> MNNTEENIDRIQEPTREDIDRKEAERLLDEAFNPRTKPVDRKKIINSALKILIGLYKEKKDDLTSASFISIARAYYLVSITILPKGTTIPEKKKEALRKGIEFIDRAINKFNGSILDSQRAFRIKSVLSIEFNRIDREKCDNIKLKNLLNEAVDKGCTDFDTYEWDIQIAIRLCELGVDMEGHFDNLIKSNKANDLQKAKAYYFIKKDDHKAKEHMDKCTASLKYTPCSHRLWDETVGFIERLKGDSSTLWRDFAIKTYRSCRVQEKETGTLRLRWYWSRHRVLYDMAFLAV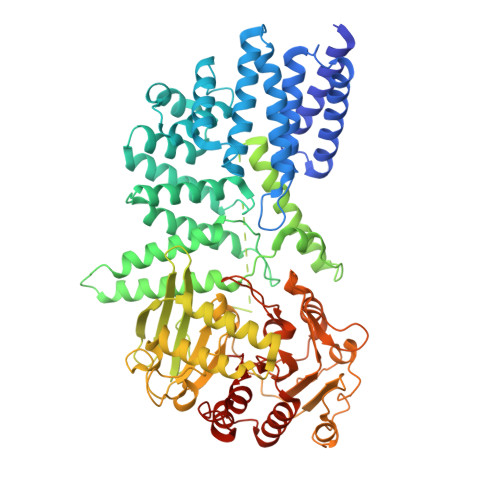KEQADDEEPDVNVKQAKIKKLAEISDSLKSRFSLRLSDMEKMPKSDDESNHEFKKFLDKCVTAYQDGYVINRSEDKEGQGENKSTTSKQPEPRPQAKLLELTQVPEGWVVVHFYLNKLEGMGNAIVFDKCANSWQYKEFQYKELFEVFLTWQANYNLYKENAAEHLVTLCKKIGETMPFLFCDNFIPNGKDVLFVPHDFLHRLPLHGSIENKTNGKLFLENHSCCYLPAWSFASEKEASTSDEYVLLKNFDQGHFETLQNNQIWGTQSVKDGASSDDLENIRNNPRLLTILCHGEANMSNPFRSMLKLANGGITYLEILNSVKGLKGSQVILGACETDLVPPLSDVMDEHYSVATALLLIGAAGVVGTMWKVRSNKTKSLIEWKLENIEYKLNEWQKETGGAAYKDHPPTFYRSIAFRSIGFPL Hydroxymethyl-pterin pyrophosphokinase (HPPK) is one such enzyme, responsible for catalysing the transfer of a pyrophosphate group from the ATP to the pterin substrate, 6-hydroxymethyl-7,8-dihydropterin (HMDP). All have a thioredoxin-like fold containing the binding sites for both the substrate and the ATP cofactor. X-ray structural studies have revealed that major conformational changes, particularly in loop L3, occur throughout the catalytic cycle. The pterin stacks between two highly conserved aromatic residues (Tyr or Phe) and both the substrate and cofactor are fixed in position by a multitude of hydrogen bonds; in total, they interact with 26 separate residues.

To investigate the factors contributing to the free energy of binding, we solved the structure of SaHPPK in complex with 21a. Attempts were made to co-crystallize each of the strongest binding compounds (21a and 21c–21e) with SaHPPK, however diffraction quality crystals could only be obtained for compound 21a. These provided excellent quality electron density data, and a high-resolution X-ray structure (1.85 Å) of the SaHPPK/21a binary complex determined via molecular replacement (crystal data and details of the data collection and refinement are provided in Table 3). The ethyl alcohol pendant projects into the space leading towards the Mg2+ binding site, making two hydrogen bond contacts with a pair of bound water molecules. 7 in the SaHPPK/8-MG structure has been displaced in the SaHPPK/21a structure, and there is a tightly bound water between the hydroxyethyl and Asp97 which orients Asp97 in a similar position to that found of Asp97 of the EcHPPK/AMPCPP/HMDP structure (where Mg2+ sits). It should be noted, however, that in contrast to 8-MG, the binding of compounds 21a, 21c and 21d was found to be 10-15-fold weaker under saturating ATP conditions, suggesting extensions from ring B into the space towards the Mg2+ centres and the ATP binding site leads to competitive binding with the ATP cofactor. Titration of 21a into 15N-labelled apo (data not shown) and magnesium-loaded SaHPPK enzyme led to broadening and disappearance of several, common peaks in the 2D 15N HSQC NMR spectrum, which is characteristic of the intermediate exchange timescale, and indicates that binding of 21a is not magnesium-dependent. This is similar to what was observed for the binding of 8-MG to SaHPPK and is consistent with the fact that density characteristic of magnesium was not observed in the X-ray crystal data of the SaHPPK/21a complex. While the spectra appear to be very similar, however, closer inspection reveals that the sidechain Hε1–Nε1 peak of Trp89 (in loop L3) is only perturbed in the 8-MG bound spectrum. This is mechanistically interesting and may indicate that this region of loop L3, adjacent to the substrate-binding loop L2, is involved in binding of 8-MG but not 21a.

>[2x]GSHMIQAYLGLGSNIGDRESQLNDAIKILNEYDGISVSNISPIYETAPVGYTEQPNFLNLCVEIQTTLTVLQLLECCLKTEECLHRIRKERWGPRTLDVDILLYGEEMIDLPKLSVPHPRMNERAFVLIPLNDIAANVVEPRSKLKVKDLVFVDDSVKRYK>PKFFYIKSELNGKVLDIEGQNPAPGSKIITWDQKKGPTAVNQL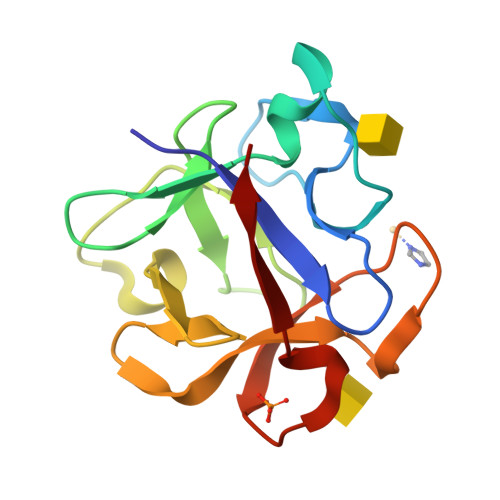WYTDQQGVIRSKLNDFAIDASHEQIETQPFDPNNPKRAWIVSGNTIAQLSDRDIVLDIIKSDKEAGAHICAWKQHGGPNQKFIIESE[2x]>MDIPKDRFYT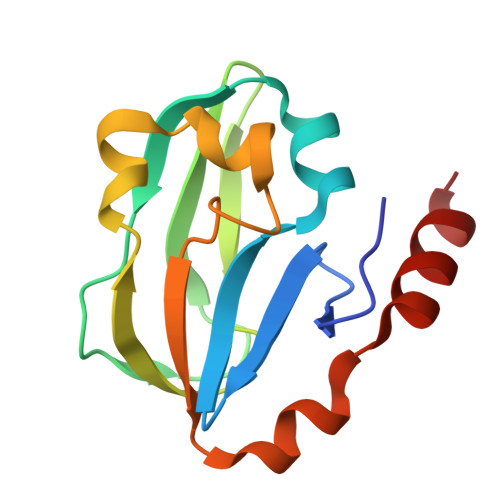KTHEWALPEGDTVLVGITDYAQDALGDVVYVELPEVGRVVEKGEAVAVVESVKTASDIYAPVAGEIVEVNLALEKTPELVNQDPYGEGWIFRLKPRDMGDLDELLDAGGYQEVLESEA[3x]>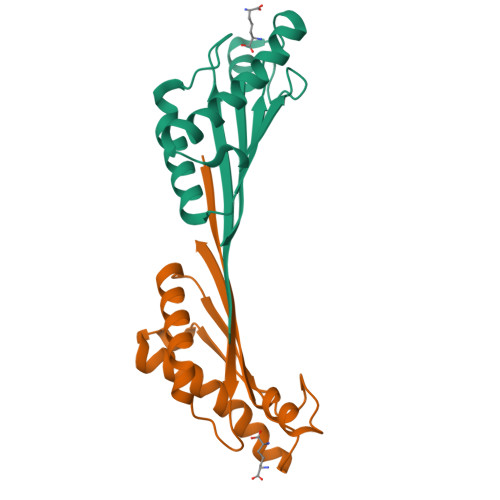[8x]GSHMELTEDLNMELRVFFDTNKSNIKDQYKPEIAKVAEKLSEYPNATARIEGHTDNTGPRKLNERLSLARANSVKSALVNEYNVDASRLSTQGFAWDQPIADNKTKEGRAMNRRVFATITGSR>[6x]MAPKSSSSGSKKKSSASSNSADAKASKFKLPAEFITRPHPSKDHGKETCTAYIHPNVLSSLEINPGSFCTVGKIGENGILVIARAGDEEVHPVNVITLSTTIRSVGNLILGDRLELKKAQVQPPYATKVTVGSLQGYNILECMEEKVIQKLLDDSGVIMPGMIFQNLKTKAGDESIDVVITDASDDSLPDVSQLDLNMDDMYGGLDNLFYLSPPFIFRKGSTHITFSKETQANRKYNLPEPLSYAAVGGLDKEIESLKSAIEIPLHQPTLFSSFGVSPPRGILLHGPPGTGKTMLLRVVANTSNAHVLTINGPSIVSKYLGETEAALRDIFNEARKYQPSIIFIDEIDSIAPNRANDDSGEVESRVVATLLTLMDGMGAAGKVVVIAATNRPNSVDPALRRPGRFDQEVEIGIPDVDARFDILTKQFSRMSSDRHVLDSEAIKYIASKTHGYVGADLTALCRESVMKTIQRGLGTDANIDKFSLKVTLKDVESAMVDIRPSAMREIFLEMPKVYWSDIGGQEELKTKMKEMIQLPLEASETFARLGISAPKGVLLYGPPGCSKTLTAKALATESGINFLAVKGPEIFNKYVGESERAIREIFRKARSAAPSIIFFDEIDALSPDRDGSSTSAANHVLTSLLNEIDGVEELKGVVIVAATNRPDEIDAALLRPGRLDRHIYVGPPDVNARLEILKKCTKKFNTEESGVDLHELADRTEGYSGAEVVLLCQEAGLAAIMEDLDVAKVELRHFEKAFKGIARGITPEMLSYYEEFALRSGSSS

The type II AAA + ATPase Drg1 is a ribosome assembly factor, functioning to release Rlp24 from the pre-60S particle just exported from nucleus, and its activity in can be inhibited by a drug molecule diazaborine. Here, we report Drg1 structures in different nucleotide-binding and benzo-diazaborine treated states. All structures display a typical three-layered architecture, similar to those of type II AAA + hexamers, such as p97/VCP and Cdc48, and the NTD, D1, and D2 rings show an apparent deviation from a perfect sixfold symmetry. Comparisons of these structures indicate that Drg1 hexamers transit between two extreme conformations, a planar and a helical state.

To understand the structural dynamics of S. cerevisiae Drg1 hexamer, we assembled Drg1 hexamers in vitro in the presence of excessive ADP or AMPPNP (a non-hydrolysable analog of ATP). To better understand the structural dynamics of Drg1 hexamers related to the nucleotide hydrolytic cycle, we analyzed the structures of Drg1 hexamers obtained from three different samples (ADP, AMPPNP, ADP/AMPPNP/benzo-diazaborine). In these datasets, only a small fraction of particles displays an approximate six-fold symmetry. Most 3D classes adopt asymmetrical conformations, with one or two subunits more flexible than others. An intriguing observation is that the nucleotide binding pockets of D1 domains in the structures of different datasets are all occupied, either by ATP or AMPPNP, even for the Drg1-ADP sample. Although the structure from the Drg1-ADP dataset was not resolved at atomic resolution, but the local densities suggest the presence of ATP in these D1 sites. Therefore, this co-purification of ATP with Drg1 implies that the D1 ATPase site likely has a high affinity for ATP and a low hydrolysis activity. There is no obvious nucleotide occupation in the D2 domains of the structures from the ADP and AMPPNP treated samples.>AVTGDTDQPIHIESDQQSLDMQGNVVTFTGNVIVTQGTIKINADKVVVTRPGGEQGKEVIDGYGKPATFYQMQDNGKPVEG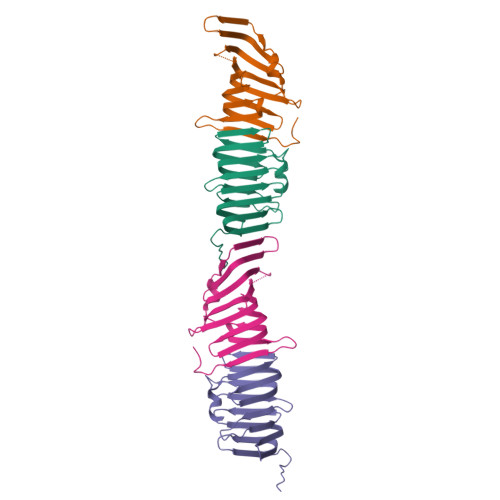HASQMHYELAKDFVVLTGNAYLQQVDSNIKGDKITYLVKEQKMQAFSDKGKRVTTVLVPSQLQDKNNKGQTPAQKKGN[2x]>[2x]MVVKAAGLVIYRKLAGKIEFLLLQASYPPHHWT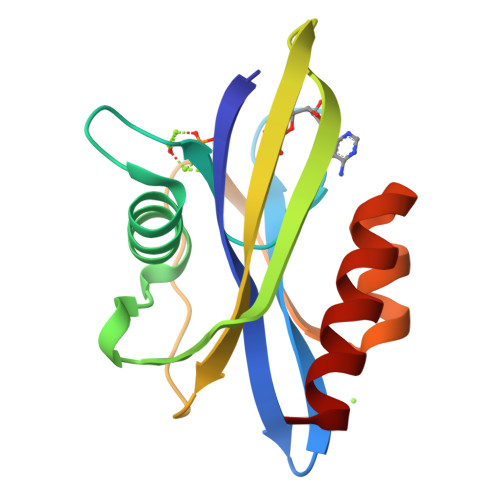PPKGHVDPGEDEWQAAIRETKEEANITKEQLTIHEDCHETLFYEAKGKPKSVKYWLAKLNNPDDVQLSHEHQNWKWCELEDAIKIADYAEMGSLLRKFSAFLAGF Gram-positive pili differ from those of Gram-negative bacteria by the presence of covalently linked subunits containing a conserved LPXTG motif or a variant of it. In S. pneumoniae, the genes coding for the pilus are contained in a 12 Kb pathogenicity island (the rlrA islet), consisting of seven genes of which rrgA, rrgB, and rrgC encode LPXTG-containing proteins. Only RrgB is strictly necessary for the pilus formation while the other two are ancillary proteins. Here the crystal structure of the RrgBD2–D4 backbone subunit fitted into the EM reconstruction of the S. pneumoniae pilus reveals for the first time the polymeric architecture of a Gram-positive pilus indicating a head-to-tail organization of individual backbone subunits.

A further crystal form designated RrgBD2–D3 (residues 141–592) was also derived via the construct design process. Crystals grown from these constructs belong to the monoclinic (space group C2) crystal form and diffracted to high resolution but lacked any ordered electron density outside regions defining domains D2 and D3. Because of the close packing of the molecules in this crystal form, it seems very likely that crystal growth occurred after a degradation event during the crystallization process. The first 262 residues (184–446) form a dual domain (D2 and D3) made of two β-sandwiches of approximately 100 residues present in all crystal forms. The C-terminal β-sheet of domain D3 contributes one additional strand to domain D2 completing the 4-stranded β-sheet of the β-sandwich. Domains D2 and D3 are oriented together in such a way that the six loops form a flat relatively broad surface of >5000 Å2. The helical component in domain D2, one 3–10 helix and a short 6 residue stretch (aa 283–289), is consistent with that found in the eukaryotic IgG immunoglobulin fold.

> AKPKIDKDFKGKANPDTPRVDKDTPVNHQVGDVVEYEIVTKIPALANYATANWSDRMTEGLAFNKGTVKVTVDDVALEAGDYALTEVATGFDLKLTDAGLAKVNDQNAEKTVKITYSATLNDKAIVEVPESNDVTFNYGNNPDHGNTPKPNKPNENGDLTLTKTWVDATGAPIPAGAEATFDLVNAQAGKVVQTVTLTTDKNTVTVNGLDKNTEYKFVERSIKGYSADYQEITTAGEIAVKNWKDENPKPLDPTEPKVVTYG Like all Apicomplexa (the phylum to which Plasmodium belong), malaria parasites move using a substrate-dependent mechanism called gliding motility, a sophisticated substrate-dependent form of cell movement based on a macromolecular complex called the glideosome. At the glideosome core is the single-headed class XIV myosin A (PfMyoA), and short and oriented filaments of a divergent actin (PfAct1). PfMyoA is a tailless myosin consisting only of a motor domain and light chain binding domain. By solving three structural states of the PfMyoA motor domain, corresponding to three states of the motor cycle, we show how the unique class XIV N-terminal heavy chain extension and its interactions with other structural elements define motor function.

The crystal type 2 contains one molecule per asymmetric unit. It corresponds to the Pre-powerstroke (PPS) state, a state with the lever arm up and able to dock to actin with electrostatic contacts. The resolution of the PPS state is poorer, but the electron density map is of good quality and allowed the entire motor domain to be built, including loops with good refinement statistics. Second, the interaction between the Relay and the SH1-helix is mainly hydrophobic both in the PPS state and in the Rigor-like state, with the exception of an electrostatic bond between the RelayQ494 and the fulcrum SH2-SH1S691 that is present in the two states.

> MAVTNEEIKTASKIVRRVSNVEAFDKSGSVFKGYQIWTDISPTIENDPNIMFVKCVVQQGSKKEKLTVVQIDPPGTGTPYDIDPTHAWNCNSQVDPMSFGDIGLLNHTNIPCVLDFLKHRYLKNQIYTTAVPLIVAINPYKDLGNTTNEWIRRYRDTADHTKLPPHVFTCAREALSNLHGVNKSQTIIVSGESGAGKTEATKQIMRYFASSKSGNMDLRIQTAIMAANPVLEAFGNAKTIRNNNSSRFGRFMQLVISHEGGIRYGSVVAFLLEKSRIITQDDNERSYHIFYQFLKGANSTMKSKFGLKGVTEYKLLNPNSTEVSGVDDVKDFEEVIESLKNMELSESDIEVIFSIVAGILTLGNVRLIEKQEAGLSDAAAIMDEDMGVFNKACELMYLDPELIKREILIKVTVAGGTKIEGRWNKNDAEVLKSSLCKAMYEKLFLWIIRHLNSRIEPEGGFKTFMGMLDIFGFEVFKNNSLEQLFINITNEMLQKNFVDIVFERESKLYKDEGISTAELKYTSNKEVINVLCEKGKSVLSYLEDQCLAPGGTDEKFVSSCATNLKENNKFTPAKVASNKNFIIQHTIGPIQYCAESFLLKNKDVLRGDLVEVIKDSPNPIVQQLFEGQVIEKGKIAKGSLIGSQFLNQLTSLMNLINSTEPHFIRCIKPNENKKPLEWCEPKILIQLHALSILEALVLRQLGYSYRRTFEEFLYQYKFVDIAAAEDSSVENQNKCVNILKLSGLSESMYKIGKSMVFLKQEGAKILTK>ATPHINAEMGDFADVVLMPGDPLRAKYIAETFLEDAREVNNVRGMLGFTGTYKGRKISVMGHGMGIPSCSIYTKELITDFGVKKIIRVGSCGAVLPHVKLRDVVIGMGACTDSKVNRIRFKDHDFAAIADFDMVRNAVDAAK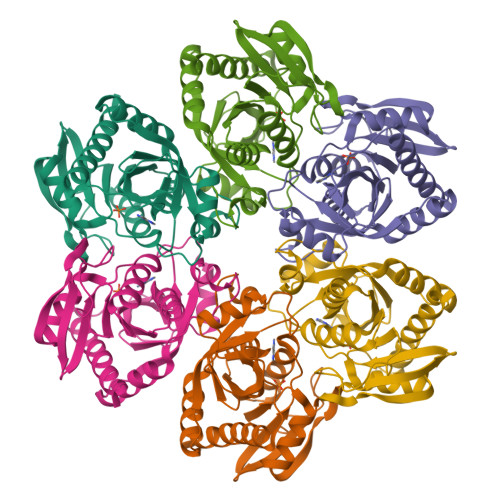ALGIDARVGNLFSADLFYSPDGEMFDVMEKYGILGVEMEAAGIYGVAAEFGAKALTICTVSDHIRTHEQTTAAERQTTFNDMIKIALESVLLGDKE[3x]4-phenyl-3-[2-(pyridin-3-yl)-1,3-thiazol-5-yl]-2,7-dihydro-6H-pyrazolo[3,4-b]pyridin-6-one | C20 H13 N5 O S | 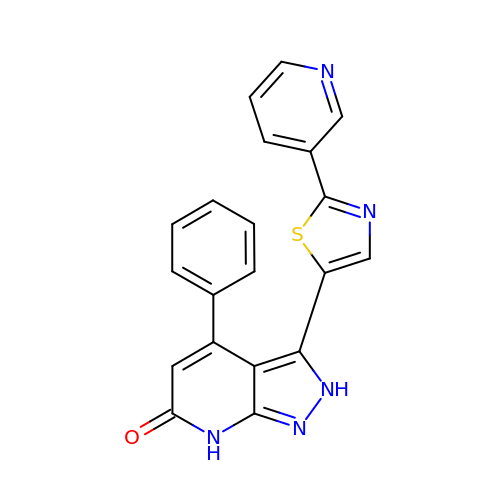GPTXKTBHBIQZEL-UHFFFAOYSA-N>[5x]GCX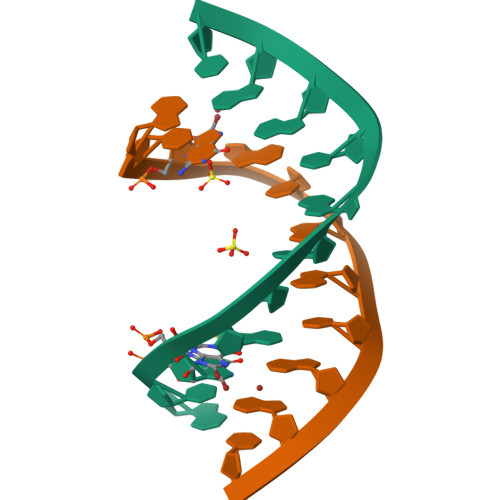GCGGCGGC> SNNLEEEVQKLLYEL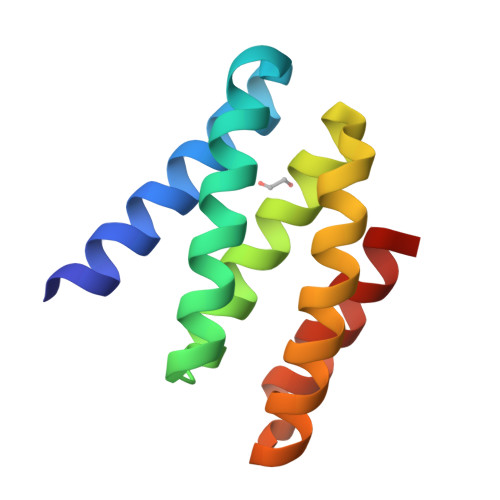SEIWHQHDHEASREALHRVLEVLKQLLEHNNLEQAVELISIAVHVAVRVNNEHVIRELHHLLRRLLKQVKEHNNNKLYIAVMSVIMQLERT> SSESIRMVLIGPPGAGKGTQAPNLQERFHAA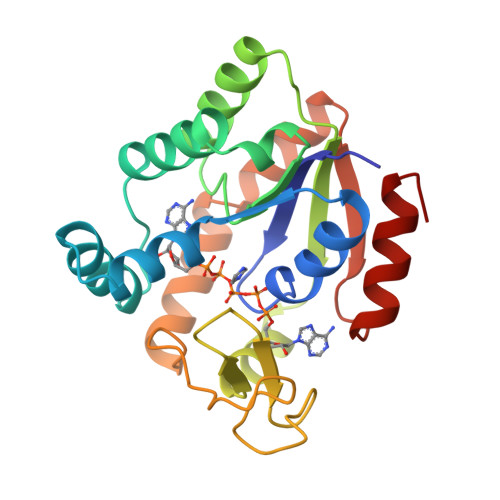HLATGDMLRSQIAKGTQLGLEAKKIMDQGGLVSDDIMVNMIKDELTNNPACKNGFILDGFPRTIPQAEKLDQMLKEQGTPLEKAIELKVDDELLVARITGRLIHPASGRSYHKIFNPPKEDMKDDVTGEALVQRSDDNADALKKRLAAYHAQTEPIVDFYKKTGIWAGVDASQPPATVWADILNKLGKN> GHMQQSDKTALTVIRLGGIFSRRQQYQLPVNVTASTLTLLLQKPLKLHDMEVVHISFERSALEQWLSKGGEIRGKLNGIGFAQKLNLEVDSAQ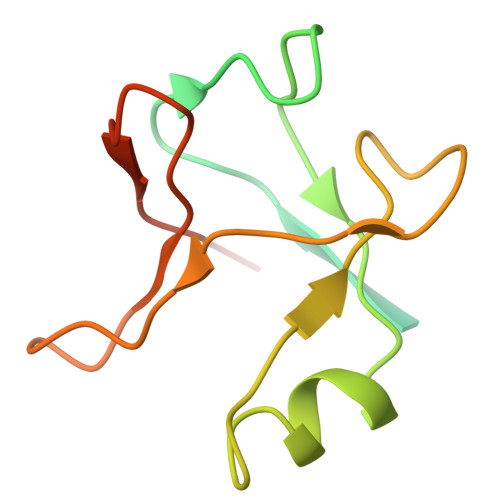HLVVRDVSLQGSTLALPGSSAE>[2x]SMAKIIFPEDF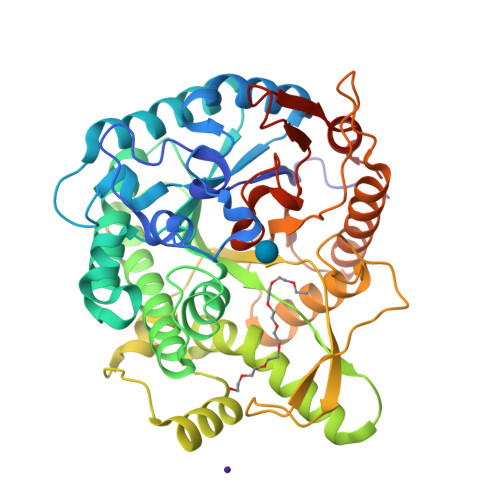IWGAATSSYQIEGAFNEDGKGESIWDRFSHTPGKIENGDTGDIACDHYHLYREDIELMKEIGIRSYRFSTSWPRILPEGKGRVNQKGLDFYKRLVDNLLKANIRPMITLYHWDLPQALQDKGGWTNRDTAKYFAEYARLMFEEFNGLVDLWVTHNEPWVVAFEGHAFGNHAPGTKDFKTALQVAHHLLLSHGMAVDIFREEDLPGEIGITLNLTPAYPAGDSEKDVKAASLLDDYINAWFLSPVFKGSYPEELHHIYEQNLGAFTTQPGDMDIISRDIDFLGINYYSRMVVRHKPGDNLFNAEVVKMEDRPSTEMGWEIYPQGLYDILVRVNKEYTDKPLYITENGAAFDDKLTEEGKIHDEKRINYLGDHFKQAYKALKDGVPLRGYYVWSLMDNFEWAYGYSKRFGLIYVDYENGNRRFLKDSALWYREVIEKGQVEAN> NDWL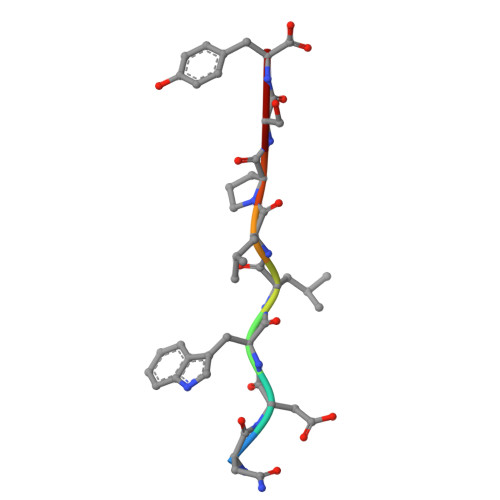LPSY>GSSGSSGPFYTQGDSLTSEDHLDDTWVTVFGFPQASASYILLQFAQYGNILKHVMSNTGNWMHIRYQSKLQARKALSKDGRIFGESIMIGVKPCIDKNVMENSDRGVLSS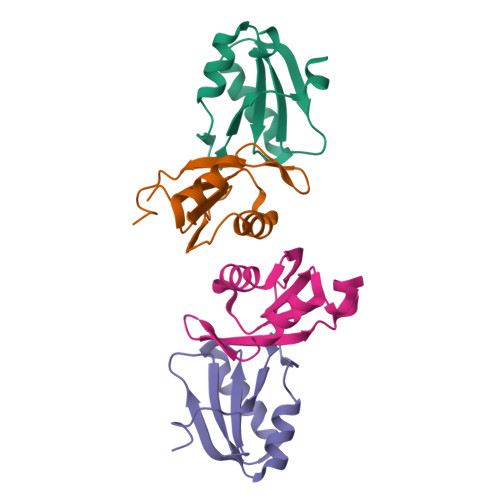PSLSGPSSG[4x]> GSAKDPKKRPENKPFDAFISYSEHDADWTKEHLLKKLETDGFKICYHERDFKPGHPVLGNIFYCIENSHKVLFVLSPSFVNSCWCQYELYFAEHRVLDENQDSLIMVVLEDLPPDSVPQKFSKLRKLLKRKTYLKWSPEEHKQKIFWHQLAAVLKTTNEPLVRAENGPNEDVIEME

TLR15 is a TLR unique to birds and reptiles that responds to virulence-associated fungal and bacterial proteases. The ectodomain of a TLR directly senses a PAMP and the intracellular TIR domain dimerizes to initiate a signaling cascade. Collectively, our structural and mutational analyses suggest that TLR15TIR employs the BB, αC2 and DD regions for dimerization.

To provide the structural mechanism whereby TLR15 mediates signaling via its intracellular TIR domain, chicken TLR15TIR (residues 699–868) was expressed using the E. coli expression system and purified by chromatographic methods in the presence of β-mercapto­ethanol. The TLR15TIR protein was crystallized using ammonium sulfate at pH 6.5. The TLR15TIR crystals diffracted X-rays up to 1.90 Å resolution. The crystal structure of TLR15TIR was determined by molecular replacement and refined with an R free value of 23.3%. Given that β-mercapto­ethanol was used for the purification of TLR15TIR and resembles the curved linear shape of the extra electron density, the Cys777 residue was modeled as an adduct with β-mercapto­ethanol. Because the TLR15 Cys777 residue is readily modified by β-mercapto­ethanol or gluta­thione, we propose that the Cys777 residue is highly reactive.>[2x]GPHMSDHKFLTQAVEEAYKGVDCGDGGPFGAVIVHNNEVVASCHNMVLKYTDPTAHAQVTAIREACKKLNKIELSECEIYASCEPCPMCFGAIHLSRLKRLVYGAKAEAAIA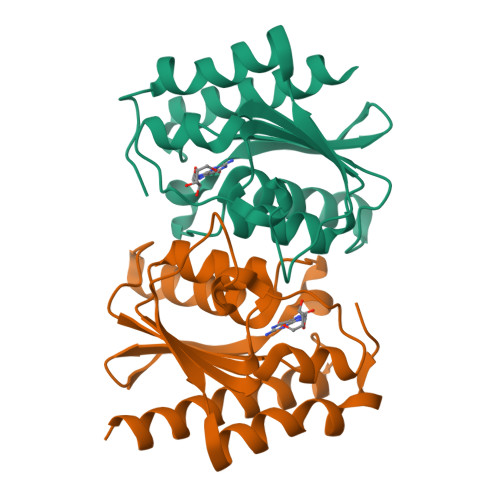IGFDDFIADALRGTGVYQKSSLEIKKADGNGAAIAEQVFQNTKEKFRLY> MKLDIKKTFSNRSDRVKGIDFHPTEPWVLTTLYSG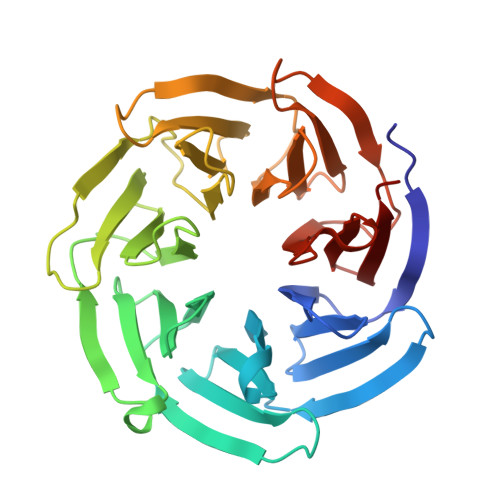RVEIWNYETQVEVRSIQVTETPVRAGKFIARKNWIIVGSDDFRIRVFNYNTGEKVVDFEAHPDYIRSIAVHPTKPYVLSGSDDLTVKLWNWENNWALEQTFEGHEHFVMCVAFNPKDPSTFASGCLDRTVKVWSLGQSTPNFTLTTGQERGVNYVDYYPLPDKPYMITASDDLTIKIWDYQTKSCVATLEGHMSNVSFAVFHPTLPIIISGSEDGTLKIWNSSTYKVEKTLNVGLERSWCIATHPTGRKNYIASGFDNGFTVLSLA>[2x]VIEKVQHIQLLQKNVRAQLVDMKRLEVDIDIKIRSCRGSC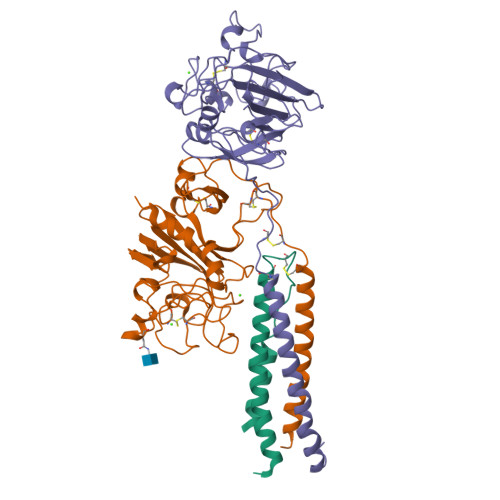SRALAREVDLKDYEDQQKQLEQVIAK;>HQLYIDETVNSNIPTNLRVLRSILENLRSKIQKLESDVSAQMEYCRTPCTVSCNIPVVSGKECEEIIRKGGETSEMYLIQPDSSVKPYRVYCDMNTENGGWTVIQNRQDGSVDFGRKWDPYKQGFGNVATNTDGKNYCGLPGEYWLGNDKISQLTRMGPTELLIEMEDWKGDKVKAHYGGFTVQNEANKYQISVNKYRGTAGNALMDGASQLMGENRTMTIHNGMFFSTYDRDNDGWLTSDPRKQCSKEDGGGWWYNRCHAANPNGRYYWGGQYTWDMAKHGTDDGVVWMNWKGSWYSMRKMSMKIRPFFPQQ[2x];>[2x]YEASILTHDSSIRYLQEIYNSNNQKIVNLKEKVAQLEAQCQEPCKDTVQIHDITGKDCQDIANKGAKQSGLYFIKPLKANQQFLVYCEIDGSGNGWTVFQKRLDGSVDFKKNWIQYKEGFGHLSPTGTTEFWLGNEKIHLISTQSAIPYALRVELEDWNGRTSTADYAMFKVGPEADKYRLTYAYFAGGDAGDAFDGFDFGDDPSDKFFTSHNGMQFSTWDNDNDKFEGNCAEQDGSGWWMNKCHAGHLNGVYYQGGTYSKASTPNGYDNGIIWATWKTRWYSMKKTTMKIIPFNRLTIGEGQQHHLGGAK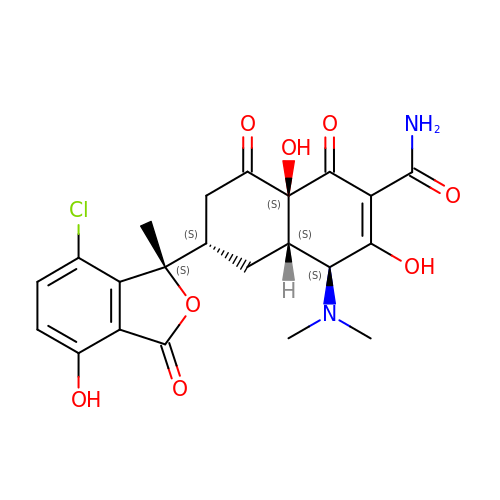ISO-7-CHLORTETRACYCLINE | C22 H23 Cl N2 O8 | GFSLIMZISCAANG-AXVXPIMKSA-N>MASGMIVTDAGADQPIVFVNRAFSTITGYAPNEVLGRNARFLQGPQTDAATVARLREAIAAARPIQERILNYRKDGQPFWNQLSISPVRDETGNVVAFV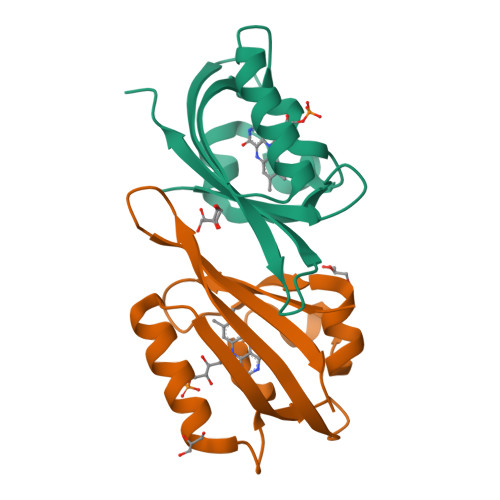GVQTDVTAHHHHHH[2x]>[8x]SMSYESPFHLNDAVAIVTGAAAGIGRAIAGTFAKAGASVVVTDLKSEGAEAVAAAIRQAGGKAIGLECNVTDEQHREAVIKAALDQFGKITVLVNNAGGGGPKPFDMPMSDFEWAFKLNLFSLFRLSQLAAPHMQKAG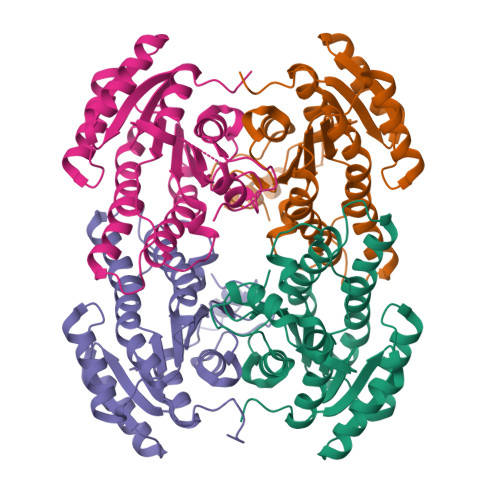GGAILNISSMAGENTNVRMASYGSSKAAVNHLTRNIAFDVGPMGIRVNAIAPGAIKTDALATVLTPEIERAMLKHTPLGRLGEAQDIANAALFLCSPAAAWISGQVLTVSGGGVQELD>AKKIFKPEELRQALMPTLEALYRQDPESLPFRQPVDPQLLGIPDYFDIVKSPMDLSTIKRKLDTGQYQEPWQYVDDIWLMFNNAWLYNRKTSRVYKYCSKLSEVFEQEIDPVMQSLGYCCGRKLEFSPQTLCCYGKQLCTIPRDATYYSYQNRYHFCEKCFNEIQGESVSLGDDPSQPQTTINKEQFSKRKNDTLDPELFVECTECGRKMHQICVLHHEIIWPAGFVCDGCLKKSARTRKENKFSAKRLPSTRLGTFLENRVNDFLRRQNHPESGEVTVRVVHASDKTVEVKPGMKARFVDSGEMAESFPYRTKALFAFEEIDGVDLCFFGMHVQEYGSDCPPPNQRRVYISYLDSVHFFRPKCLRTAVYHEILIGYLEYVKKLGYTTGHIWACPPSEGDDYIFHCHPPDQKIPKPKRLQEWFKKMLDKAVSERIVHDYKDIFKQATEDRLTSAKELPYFEGDFWPNVLEESIKELEQEEEERKREENTGNKKKPGMPNVSNDLSQKLYATMEKH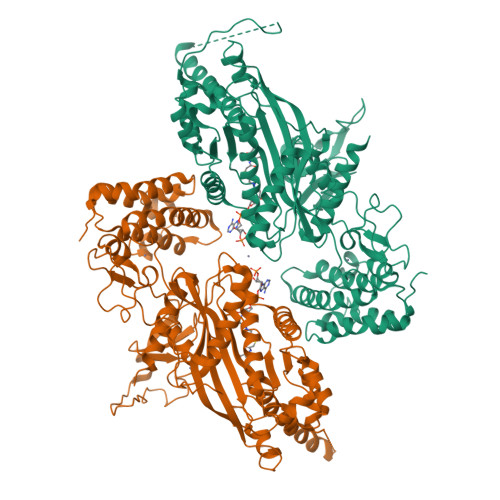KEVFFVIRLIAGPAANSLPPIVDPDPLIPCDLMDGRDAFLTLARDKHLEFSSLRRAQWSTMCMLVELHTQSQD[4x]(6S)-6-(2-tert-butoxy-2-oxoethyl)-4-(4-chlorophenyl)-2,3,9-trimethyl-6,7-dihydrothieno[3,2-f][1,2,4]triazolo[4,3-a][1,4]diazepin-10-ium 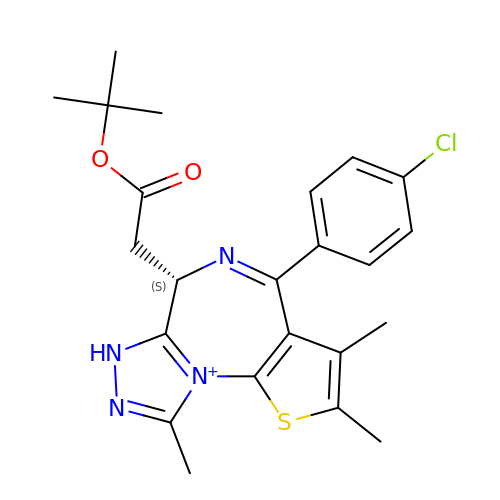| C23 H26 Cl N4 O2 S | DNVXATUJJDPFDM-KRWDZBQOSA-O> MRFKKHVVQHEETMQAIAQRYYGDVSYWIDLVEHNNLKYPYLVETDEEKMKDPERLASTGDTLIIPIESDLTDVSAKE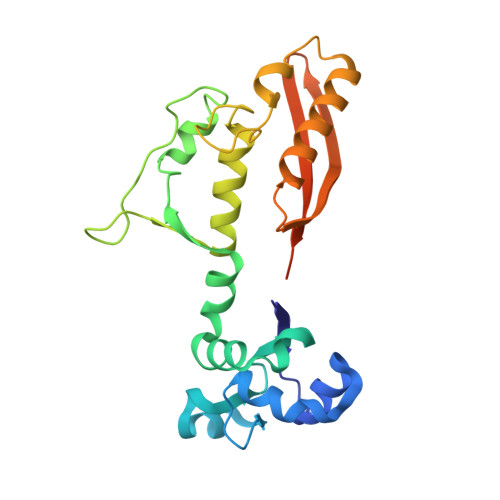INSRDKDVLVELALGRDLNITADEKYFNEHGTSDNILAFSTNGNGDLDTVKGIDNMKQQLQARLLTPRGSLMLHPNYGSDLHNLFGLNIPEQATLIEMEVLRTLTSDNRVKSANLIDWKIQGNVYSGQFSVEIKSVEESINFVLGQDEEGIFALFE> QGPDSMKKDVPPSINTTNIDTLLVATDQTERIVEPPENIQEKIAFIFNNLSQSNMTQKVEELKETVKEEFMPWVSQYLVMKRVSIEPNFHSLYSNFLDTLKNPE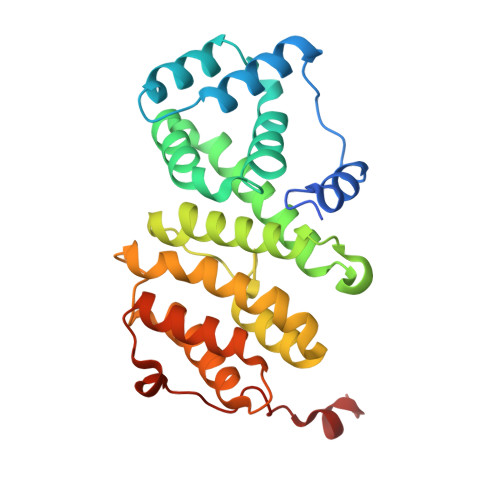FNKMVLNETYRNIKVLLTSDKAAANFSDRSLLKNLGHWLGMITLAKNKPILHTDLDVKSLLLEAYVKGQQELLYVVPFVAKVLESSIRSVVFRPPNPWTMAIMNVLAELHQEHDLKLNLKFEIEVLCKNLALDINELKPGNLLKDKDRLKNLDE>[2x]SNAMSKVLVLKSSILATSSQSNQLADFFVEQWQAAHAGDQITVRDLAAQPIPVL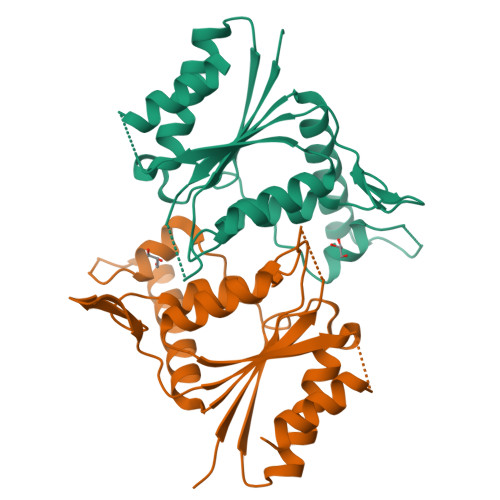DGELVGALRPSGTALTPRQQEALALSDELIAELQANDVIVIAAPMYNFNIPTQLKNYFDMIARAGVTFRYTEKGPEGLVTGKRAIILTSRGGIHKDTPTDLVVPYLRLFLGFIGITDVEFVFAEGIAYGPEVATKAQADAKTLLAQVVAA>[8x]MSTHSSTVQNDLAALIHPNTNLAQHREVGPLVIARGDGVRVFDEQGNAYIEAMSGLWSAALGFSEQRLVDAAVEQFKQLPYYHSFSHKTNAPAAALAAKLAALAPGDLNHVFFTNSGSEANDSVVKMVWYVNNALGRPAKKKFISRQQAYHGATVAAASLTGIPSMHRDFDLPAIPVHHLTCPNFYRFARPGESQEAFTVRLANELERYILAEGPETIAAFIGEPVIAAGGVIPPP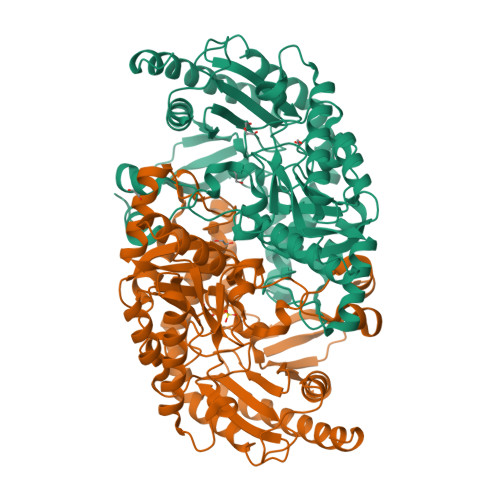TGYWAAIQAVCKRYDILVVIDEIITGFGRLGTMFGSQLYGIQPDIMVLSKQLTSSYQPLAAVVVSDAMNDVLVSQSQRLGAFAHGFTCTGHPVATAVALENIRIIEERDLVGHVQHLAPVFQRHLRAFEDHPLVGNVRGVGLMGGIELVADKATRQPFAQPGTLGGYVFKQAHKHGLIIRAIYDTIAFCPPLITTQDDIEAIFSAFERTLADATDWARSQHLL>[5x]MTVTYTARVAKARFGGFSKLLLLWRGSIYKLLWRELLCFLGLFMALSAAYRFVLTEEQKRYFEKLVLYCDRYASLIPVSFVLGFYVTLVVHRWWNQYLSMPLTDALMCVVVGTVHGHDERGRLYRRTLMRYAGLSGVLILRSVSTAVFKRFPTIDHVVEAGFMTREERKKFENLNSSYNKYWVPCVWFCNLAAQARREGRIRDNGAFKLLLEELNVFRSKCGMLFHYDWISVPLVYTQVVTIAVYSYFLACLIGRQFLDPAQGYKDHDLDLCVPIFTLLQFFFYAGWLKVAEQLINPFGEDDDDFETNFLIDRCFQVSMLAVDEMYDDLAMLEKDLYWDAAEARA

Bestrophin-1 (Best1) and bestrophin-2 (Best2) are two members of the bestrophin family of calcium (Ca2+)-activated chloride (Cl−) channels with critical involvement in ocular physiology and direct pathological relevance. The bestrophins are a family of Ca2+-activated anion channels consisting of four members (Best1–4) in mammals. The overall architecture of hBest1 and hBest2 resembles the pentameric assembly previously shown by KpBest, cBest1 and bBest2, and retains the two landmark permeation constrictions, the neck and aperture, in the ion conducting pathway. Ample electrophysiological evidence indicates that the neck and aperture serve as dual Ca2+-dependent channel “gates”, as disrupting either of them partially impairs Ca2+-dependence while disrupting both makes the channel completely Ca2+-independent.

To further investigate the structural significance of the AS, we generated hBest11–345 and bBest21–345, and solved their structures in the presence of 5 mM Ca2+ at 2.4 Å and 1.9 Å, respectively. Remarkably, both structures exhibited 100% of particles with a fully open neck, in sharp contrast to the only ~10% particles with partially or fully open neck in WT hBest1 and hBest2, respectively. Previously, we found that bBest21–406 conducts similar Cl− currents to those from the full-length bBest212, suggesting an insignificant role of the residues after position 406 in channel gating. Remarkably, removing the AS from hBest1 and hBest2 results in truncation mutants that both exhibit a fully open neck in 100% of Ca2+-bound particles in cryo-EM and conduct indistinguishable and significantly elevated currents in patch clamp, while swapping the AS between hBest1 and hBest2 results in chimeric mutants with exchanged channel activities.[6-methyl-4-[(3-methylsulfanylpropylamino)methyl]-5-oxidanyl-pyridin-3-yl]methyl 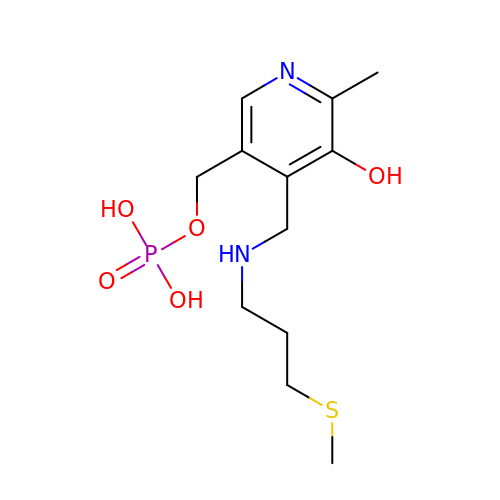dihydrogen phosphate | C12 H21 N2 O5 P S | AGFAHJKGUOFCGH-UHFFFAOYSA-N>MHHHHHHENLYFQGPNFSGNWKIIRSENFEELLKVLGVNVMLRKIAVAAASKPAVEIKQEGDTFYIKTSTTVRTTEINFKVGEEFEEQTVDGRPCKSLVKWESENK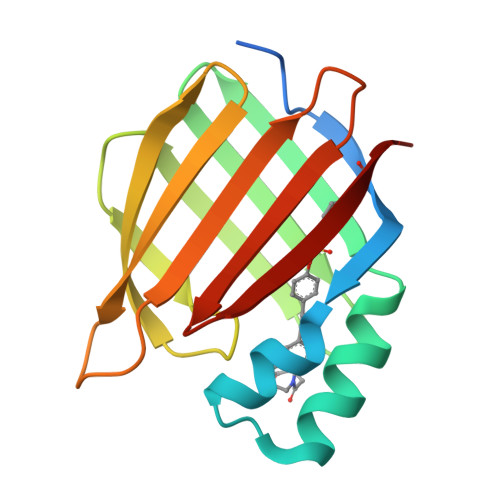MVCEQKLLKGEGPKTSWTRELTNDGELILTMTADDVVCTRVYVRE[2x]>MGSSHHHHHHSQDPNSSSMASEGVLLGMGNPLLDISCVVDDAFLEKYGLTLNNAILAEDKHLPMYKELAANPDVEYIAGGATQNTIRIAQWMLGESNATSYFGCVGKDEYGDRMFKLASEGGVNIRYDVDEDLPTGTCGVLVVKGERSLVANLSAANKYKIDHLKKPENWAFVEKAKYIYSAGFFLTVSPESMMTVAKHAAETGKYYMINLAAPFICQFFKDPLMELFPYVDFIFGNESEARAFAQVQGWETEDTKVIAVKLAALPKAGGTHKRVAVITQGTDPTIVAEDGKVTEFPVTPIPKEKLVDTNAAGDSFVGGFLSQLVLGKDIAQCVRAGNYAASVIIQRSGCTFPSKPSFESQ[2x]

Adenosine undergoes ATP-dependent phosphorylation catalyzed by adenosine kinase (ADK). In plants, ADK also phosphorylates cytokinin ribosides, transport forms of the hormone. We discovered that maize and moss enzymes can form dimers upon increasing protein concentration, setting them apart from the monomeric human and protozoal ADKs. Structural and kinetic analyses revealed a catalytically inactive unique dimer.

In contrast, both moss ADKs were observed to dimerize already at a low concentration from 0.01 mg ml–1 (0.25 µM) and became mainly dimeric (MW 81±4 kDa) above 0.3 mg ml–1 (7.7 µM). Indeed, the diameter of PpADK1 (dimeric in solution) became smaller, reaching that of the monomer and demonstrating that dimeric PpADK1 dissociates to monomers during a ternary complex formation in order to be active. The asymmetric unit contains one monomer for the ZmADK3–AP5A complex and two monomers for the PpADK1–Ado–ADP complex, all in the closed conformation. Structural comparison between ZmADK2 (open state) and the closed state of both ZmADK3 and PpADK1 reveals that AP5A (or Ado) binding induced a rigid-body motion of the smaller domain towards the large domain, resulting in the closed conformation. The electron density maps of Ado and ADP in PpADK1 show clearly that both substrates bind in the Ado- and ATP-binding sites, respectively. When superimposed, Ado in PpADK1 overlaps the Ado part of AP5A in a highly hydrophobic pocket. The purine ring of Ado stacks on the phenyl ring of Phe169 (in ZmADK3 numbering; PpADK1 numbering is shifted lower by three amino acids) and establishes hydrophobic interactions with Leu17, Ala66, Cys123, Leu134, and Ala136. The adenine part of ADP in PpADK1 is slightly shifted compared with the adenine moiety of the ATP part of AP5A due to the presence of a threonine at position 264 in PpADK1 instead of an alanine (Ala265) in ZmADK3. To form the closed ternary complex and bring the two subunits close together, the enzyme must be monomeric as shown by the structures of both ZmADK3 bound to AP5A and PpADK1 bound to ADP and Ado. We infer that dimer dissociation is likely to be the rate-limiting step in the catalysis of both moss enzymes and it is consistent with their up to 10-fold lower kinase activities compared with the predominantly monomeric maize ADKs.> MKSSHHHHHHENLYFQSNAKQALLWRDSETFILTSIELYNWGGFQGYHRAEIDPSGTAVIGPTGSGKTTLVDALMTLLCANPRYNLASTGGHESDRDLVSYVRGVTGPGDGGVEQSHIARQGKTVTAIAATLERDGAQVRLGAVLWFEGTSSSASDLKKLWLLSESPEQTLEHWLSQHHAGGMRALRQMEKDGMGIWPYPSKKAFLARLRDYFEVGENAFTLLNRAAGLKQLNSIDEIFRELVLDDRSAFERAAEVASSFDDLTDIHRELETARKQQRSLQPVADGWERYRALQEQLQDKQALEGILPVWFAEQGYRLWLAETNRLEKEHKQAELDQAQCRSQLEIQKGVVDQHRQRYLRVGGAGIDQLRGRIADWVRECDKRRLKAEQYQRLAKGLGLADELSAAALEENQQQIAARLEILAQQTTDARQKAFDAGLVQQELNGRLQSLQQERAEVERRPGSNLPGHFHAFRGDLAQELGVDESALPFVAELVQVKPEELAWRGAIERAIGSHRLRILVPQGSSQAALRWVNQRHNRLHVRLLEVKEPSSRPVFFDDGFTRKLTFKEHPYREAVKALLADNDRHCVESTEQLRHTPHAMTAQGLMSGKERFFDKQDQKRLDEDWLTGFDNRDRLAFLAEQIREVNEQLVPAKLALDAAQGDVGQLESQASLLQRIEELQFDDIDRPGAERQLQSLRTQLDTLTRPDSNLAVIKAELDQAEALRESLDQQLQRLIEQCVQLKTQFDQAASATRKAYRGAEKGLSDTQRELAQAHFPILSTDDLGDIDELERKHTRELQGQLKTLGEKLGDQKTELAKRMSDALKADTGALAEVGRELVDVPRYLERLRVLTEEALPEKLKRFLEYLNRSSDDGVTQLLSYIDHEVSMIEERLDDLNSTMQRVDFQPGRYLRLVAKKVIHESLRTLQHAQRQLNSARFIDDEGESHYKALQALV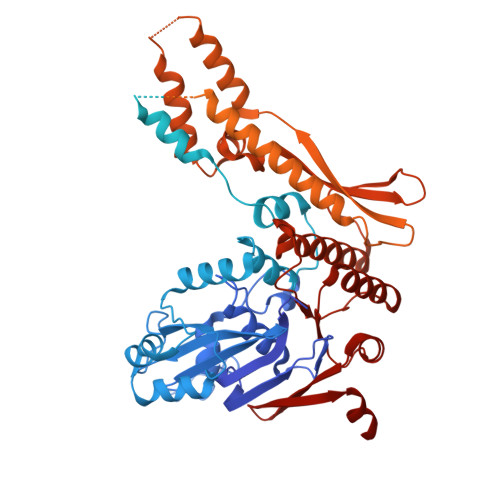GLLKDACEHSRNQGAKALLDPRFRLEFAVSVIDREGNNLIETRTGSQGGSGGEKEIIASYVLTASLSYALCPDGSSRPLFGTIVLDQAFSRSSHAVAGRIIAALREFGLHAVFITPNKEMRLLRHHTRSAVVVHRRGVESSLVSLSWEALDEHHQQRIRAMHEVAH>MRGSHHHHHHGSMKRAVITGLGIVSSIGNNQQEVLASLREGRSGITFSQELKDSGMRSHVWGNVKLDTTGLIDRKVVRFMSDASIYAFLSMEQAIADAGLSPEAYQNNPRVGLIAGSGGGSPRFQVFGADAMRGPRGLKAVGPYVVTKAMASGVSACLATPFKIHGVNYSISSACATSAHCIGNAVEQIQLGKQDIVFAGGGEELCWEMACEFDAMGALSTKYNDTPEKASRTYDAHRDGFVIAGGGGMVVVEELEHALARGAHIYAEIVGYGATSDGADMVAPSGEGAVRCMKMAMHGVDTPIDYLNSQGTSTPVGDVKELAAIREVFGDKSPAISATKAMTGHSLGAAGVQEAIYSLLMLEHGFIAPSINIEELD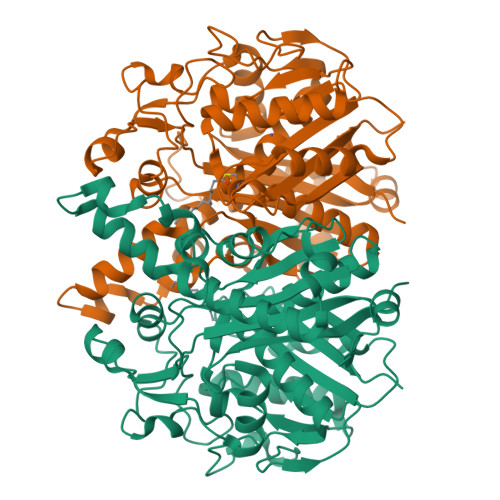EQAAGLNIVTETTDRELTTVMSNSFGFGGTNATLVMRKLKD[4x]Cytidine deaminases (CDAs) catalyze the hydrolytic deamination of cytidine and 2′-deoxycytidine to uridine and 2′-deoxyuridine. Here, we report that prokaryotic homo-tetrameric CDAs catalyze the nucleophilic substitution at the fourth position of N4-acyl-cytidines, N4-alkyl-cytidines, and N4-alkyloxycarbonyl-cytidines, and S4-alkylthio-uridines and O4-alkyl-uridines, converting them to uridine and corresponding amide, amine, carbamate, thiol, or alcohol as leaving groups. The second one is formed by the homotetrameric enzymes (T-CDA) such as CDAs from Homo sapiens and Bacillus subtilis. Both classes of CDAs contain one catalytic zinc ion per subunit. We propose that CDAs that are active toward a wide range of substrates participate in salvage and/or catabolism of variously modified pyrimidine nucleosides.

CDA_F14 was chosen as the crystallization object because of its wide substrate specificity. Asymmetric unit contained eight CDA_F14 subunits forming tetramers. Each subunit of the CDA_F14 tetramer consisted of a core of five β strands (β1 to β5) sandwiched by five α helices (α1 to α5) and exhibited a fold characteristic of the CDA family. The catalytic zinc ion in CDA_F14 was coordinated by three cysteine residues located in α helices α2 (Cys53) and α3 (Cys91 and Cys88). Three subunits were involved in the formation of the active center. In the crystal structure, the active site was occupied by two molecules of 2-methyl-2,4-pentanediol, which was used as a crystallization agent. N4-benzoyl-2′-deoxycytidine was docked into the determined structure of CDA_F14, and the following interacting residues of amino acids were found: Glu55, Asn42, Glu44, Gly54, Cys88, Tyr24, Ala46(D), and Tyr48(D). The hydrophobic substrate binding pocket area of CDA_F14 (distance to the docked substrate shorter than 3.9 Å) was formed by Val26, Ile77, Thr79, Gly85, Ala86, Pro87, Leu107, Phe126(B), and Leu131(B). The β3α3 loop (amino acids 79 to 88) of CDA_F14, connecting the third β strand to the fourth α helix, was identified as most likely to influence the space for binding of N4-substituted nucleosides. The CDA_F14 had Gly81 and Gly85 at the corresponding positions; consequently, the binding pocket of CDA_F14 was larger than that in CDA_Mmu.

>[8x]MNKEDLLKKAFEAMENAYAPYSNYHVGACALMKDGTTFLGANIENASYGATNCGERSAIFAAYSNGYRADDIEALAIVTDGDRVGAPCGICRQVLSELLNDNTPIYLSNGKETLEKTIDELLPMRFTKEDLLGHHHHHHG The African swine fever virus (ASFV) type II topoisomerase (Topo II), pP1192R, is the only known Topo II expressed by mammalian viruses and is essential for ASFV replication in the host cytoplasm. In ASFV, a functional viral Topo II pP1192R has been identified, encoded by a viral gene conserved in ASFV strains, P1192R. pP1192R is detectable at an intermediate to late stage of ASFV infection, mainly within the cytoplasmic virus factory, and has been confirmed to be important for ASFV replication. Topo IIAs exhibit a 2-fold symmetry and comprise two functional domains: an ATPase domain and a DNA binding/cleavage domain. The mechanism of enzymatic action involves the opening and closing of three gate-like dimeric interfaces, which are called the N-, DNA- and C-gate, respectively, upon ATP binding and hydrolysis and DNA cleavage that introduces a double-strand break in the DNA (G-segment) trapped in the DNA-gate for transport of another DNA strand (T-segment).

To this end, the cryo-EM sample of DNA-bound pP1192R was prepared by adding both a DNA duplex, m-AMSA, and AMP-PNP. The high quality EM map allow us to build the atomic model of the pP1192R DNA-binding/cleavage domain in complex with both DNA duplex and m-AMSA. Secondary structural elements of the protein, all the DNA base pairs, two m-AMSA molecules, and ions (presumably Mg2+ as it presents in the buffer) were well resolved. The overall configuration of the complex resembles the drug-poisoned cleavage complex of eukaryotic and prokaryotic Topo IIAs, with the C-gate adopting a closed conformation. As presented in other Topo IIA-DNA complexes, the DNA duplex was trapped in the DNA-gate and symmetrically kinked by intercalation of a proline (P852) from each protomer into the DNA minor groove at two points. In one strand, the rupture of the phosphodiester bond was observed between –1 and +1 nucleotides, with the 5′-phosphate of the +1 adenine covalently attached to catalytic tyrosine (Y800) of the cleavage active site, confirming the formation of the cleavage complex, and a m-AMSA molecule was found wedged into the DNA base pair stacks (+1/+4 and –1/+5) flanking the cleaved scissile phosphate. However, there was coherent density in the EM map of the other DNA strand, with no phosphodiester bond break was found at the expected scissile phosphate, indicating a pre-cleavage state. Moreover, an extra density appeared bridging the phenolic hydroxyl group of the Y800 and the 5′ phosphate of +1 adenine, reminiscent of the position of the metal ion A2+ proposed in the intermediate state of the classical two-metal catalysis model. Since the DNA strand is intact at Site 2 and no m-AMSA orientation consistent with that in Site 2 was found at the site of DNA strand break, we propose that m-AMSA in the Site 2-like orientation may impede the function of pP1192R by preventing DNA cleavage and stabilizing a pre-cleavage enzyme–DNA complex.

>[2x]METFEISDFKEHAKKKSMWAGALNKVTISGLMGVFTEDEDLMALPIHRDHCPALLKIFDELIVNATDHERACHNKTKKVTYIKISFDKGVFSCENDGPGIPIVKHEQASLIAKRDVYVPEVASCYFLAGTNINKAKDCIKGGTNGVGLKLAMVHSQWAILTTADGSQKYVQHINQRLDNIEPPTITPSREMFTRIELMPVYQELGYAQPLSETEQADLSAWIYLRACQCAAYVGKGTTIYYNDKPCSTSSVMALAKMYTLVTAPNSTIYTATIKADAKPYSLHPLQVAAVVSPKFKKFEHVSIINGVNCVKGEHVTFLKKAINEMVVKKFQQTIKDKNRKTTLRDSCSNIFVVIVGSIPGIEWTGQRKDELSIAENVFKTHYSIPSSFLTSMTRSIVDILLQSISKKDNHKQIDVDKYTRARNAGGKKAQDCMLLAAEGDSALSLLRAGLTLGKSNPSGPSFDFCGMISLGGVIMNACKKVTNITTDSGETIMVRNEQLTNNKVLQGIVQVLGLDFNCHYKTQEERAKLRYGCIVACVDQDLDGCGKILGLLLAYFHLFWPQLIVHGFVKRLLTPLIRVYEKGNTVPVEFYYEQEFDAWAKKQTSLANHTVKYYKGLAAHDTHEVKSMFKHFDKMVYTFTLDDSAKELFHIYFGGESELRKRELCTGVVPLTETQTQSIHSVRRIPCSLHLQVDTKAYKLDAIERQIPNFLDGMTRARRKILAGGLKCFASNNRERKVFQFGGYVADHMFYHHGDMSLNTSIIKAAQYYPGSSHLYPVFIGIGSFGSRHLGGKDAGSPRYISVQLASEFIKTMFPTEDSWLLPYVFEDGQRAEPEYYVPVLPLAIMEYGANPSEGWKYTTWARQLEDILALVRAYVDKNNPKHELLHYAIDHKITVLPLRPSNYNFKGHLKRFGQYYYSYGTYVVSEQRNMITITELPLRVPTVAYIESIKKSSNRMAFIEEIVDYSSSETIEILVKLKPNSLSRIMEEFKETEEQNSIENFLRLRNCLHSHLNFVKPKGGIIEFNSYYEILYAWLPYRRDLYQKRLMRERAVLKLRLIMETAIVRYINESADLNLSHYEDEKEAGRILSEHGFPPLNQSLITSPEFATIEELNQKALQGCYTYILSLQARELLIAAKTRRVEKIKKMQARLDKVEQLLQESPFPGASVWLEEIDAVEKAIIKGRNTQWKFHHH>[2x]MFENITAAPADPIYGLADLFRADERPGKINLGLALYYDETGKIPVLTSVKKAEQYLLENETTKLYLGIDGIPEFGRCTQELLFGKGSAL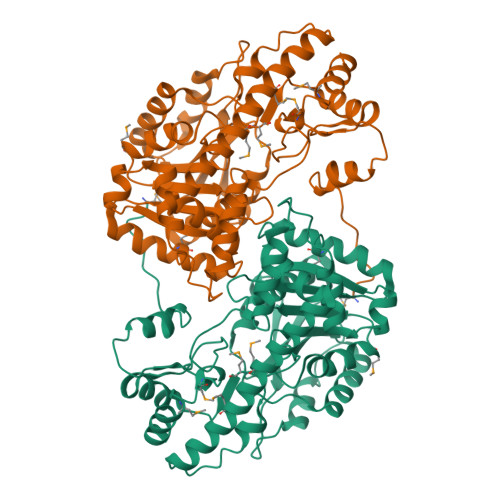INDKRARTAQTPGGHGALRVAADFLAKNTSVKRVWVYNPSSNCSKSVFNSAGLEVREYAYYDAENHTLDFDALINSLNEAQAGDVVLFTGCCHNPTGIDPTLEQWQTLAQLSVEKGWLPLFTFFYQGFARGLEEDAEGLRAFAAMHKELIVASSYSKNFGLYNESVGACTLVAADSETVDRAFSQMKAAIRDNYSSPPAHGASVVATILSNDALRAIWEQELTDMRQRIQRMRQLFVNTLQEKGANRDFSFIIKQNGMFSFSGLTKEQVLRLREEFGVYAVASGRVNVAGMTPDNMAPLCEAIVAVLGSLEHHHHHH>[2x]GAMGSTSLEPTSTLVRVRKS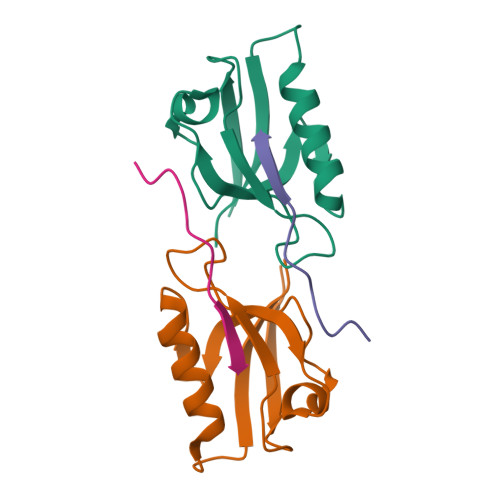AATLGIAIEGGANTRQPLPRIVTIQRGGSAHNCGQLKVGHVILEVNGQTLRGKEHKEAARIIAEAFKTKERDYIDFLVTEFN;>[2x]ERLTLPPSEITLL> IVDCGPPDDLPSGRVEYITGPGVTTYKAVIQYSCEETFYTMK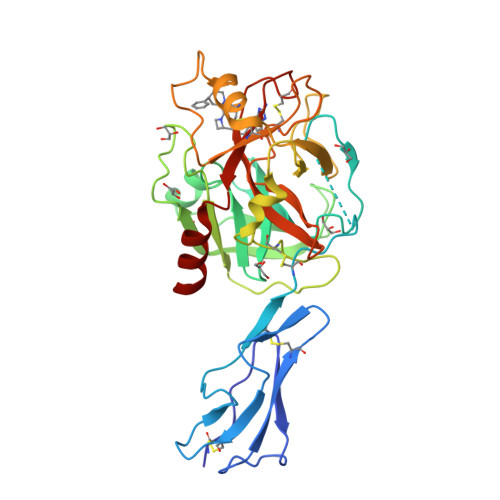VNDGKYVCEADGFWTSSKGEKSLPVCEPVCGLSARTTGGRIYGGQKAKPGDFPWQVLILGGTTAAGALLYDNWVLTAAHAVYEQKHDASALDIRMGTLKRLSPHYTQAWSEAVFIHEGYTHDAGFDNDIALIKLNNKVVINSNITPICLPRKEAESFMRTDDIGTASGWGLTQRGFLARNLMYVDIPIVDHQKCTAAYEKPPYPRGSVTANMLCAGLESGGKDSCRGDSGGALVFLDSETERWFVGGIVSWGSMNCGEAGQYGVYTKVINYIPWIENIISDF>ESPLPKPVLDTNGKELNPDSSYRIISIGRGALGGDVYLGKSPNSDAPCPDGVFRYNSDVGPSGTPVRFIPLSTNIFEDQLLNIQFNIPTVKLCVSYTIWKVGNLNAYFRTMLLETGGTIGQADNSYFKIVKSSKIGYN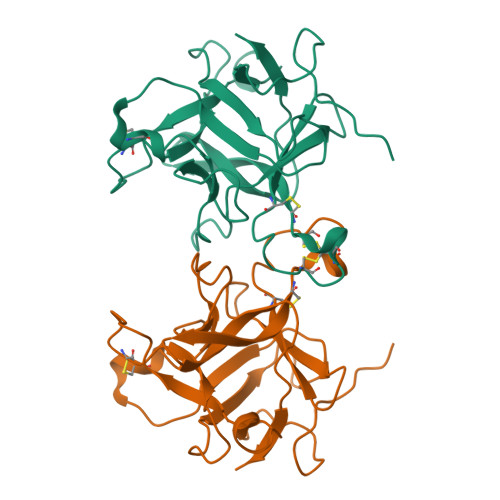LLSCPFTSIICLRCPEDQFCAKVGVVIQNGKRRLALVNENPLDVLFQEV[2x]>[2x]MKKLVLLMLVLLLVYPHVSKAGGFKGGGGNPGYWFAGDPVEHPDPAKPPIVFVHGLNGSSSAWFDENDMAEQAWKNGYDAAFI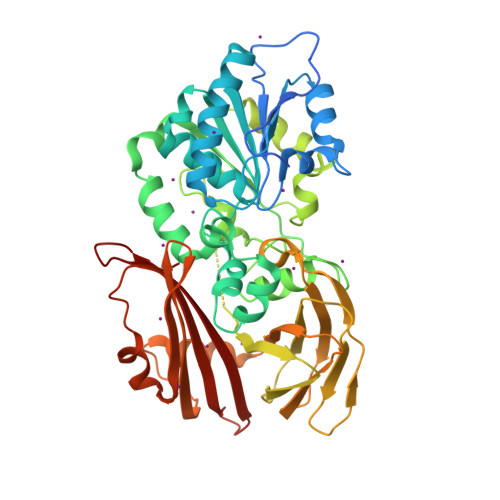DLHPDKDMQDNGAMLAAKLREIYQYFGRKVILVSYSKGGIDSQSALIHHNAYHYVERVITLGTPHHGSQLADLAYSNWAGWLADILGQKNDAVYSLQTGFMKSFRDQTDNHPNRLKTKYFTLAGNKIGGFGSALFFGGVYLNMFGENDGAVTEKNARLPYATNLDTGKWDHFSIIKGNLTFPVFMPLLTIQANANETAATKENLSYPFIRGGENHGLREEEFAVEKGVKEITVHWLSNHSSGNIKLTDPRGKPFKDFSIAKTADVFEGGFVHSAAIKNPAAGTWKIASSVKQKEAFLFIVTFDSPLNQQIKNAVTRESSNLANVKASVRSIRYENGKQAEKKSLKPASINALQNSLSFKKAGMYSVTIDLSGKTADNSPFNRTIIRSIYVNDKGEKFENSPLSD>[2x]RLSDTKAAGEVKA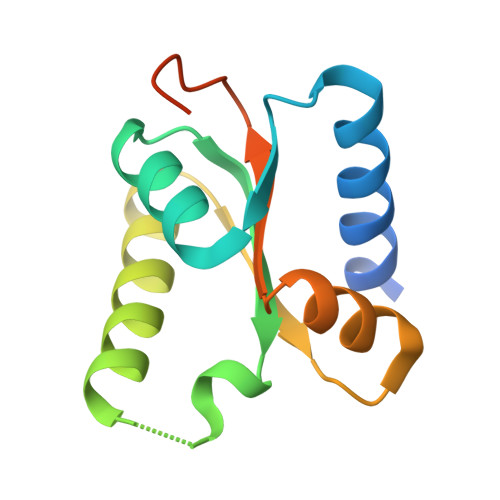LDDFYKMLQHEPDRAFYGLKQVEKANEAMAIDTLLISDELFRHQDVATRSRYVRLVDSVKENAGTVRIFSSLHVSGEQLSQLTGVAAILRFPVPELSDQEGDSSSEED ABCA4 (also known as ABCR or the rim protein) is a retinal-specific member of the ABCA subfamily predominantly expressed in the outer segment disk membranes of photoreceptor cells, and was the first ABCA transporter that has been linked to genetic disease. Available evidence suggested that ABCA4 may act as a flippase to translocate N-retinylidene-phosphatidylethanolamine (NRPE), a reversible covalent adduct of all-trans retinal (ATR) and phosphatidylethanolamine (PE), from the luminal leaflet to the cytoplasmic leaflet of the disk membrane. Here, we show the molecular structures of human ABCA4 determined in three distinct functional states by single-particle cryo-EM to 3.3–3.4 Å. These structures delineate the conformational transitions of ABCA4 to flip NRPE and suggest a “lateral access and extrusion” mechanism for ABCA4-mediated NRPE recognition and translocation, a mechanism that might also be adopted by other ABCA transporters.

To visualize ATP-driven conformational rearrangements of ABCA4, we characterized the structure of ABCA4QQ, a mutation that abolished ATP hydrolysis but maintained ATP binding, in the presence of 10 mM ATP/Mg2+. The structure was resolved at an overall resolution of 3.3 Å, showing excellent side-chain density for most of the protein except the lid and RD regions. Two strong and well-defined EM densities were observed for two bound ATP-Mg2+ molecules that were sandwiched between the two NBDs. The two NBDs exhibit a typical “head-to-tail” configuration predicted for all ABC transporters, forming two ATP binding-sites between the Walker A motif of one NBD and the ABC signature motif of the other NBD. The V-shaped lateral-opening conformation of the TMDs in the nucleotide-free ABCA4 structures is completely altered upon NBD dimerization induced by ATP binding. The two TMDs in the ATP-bound state form a closed conformation owing to the extensive interactions between TMs 1/2/5 and TMs 7/8/11, in contrast to a narrow interface in the cytoplasmic membrane leaflet between TM5 and TM11 in the nucleotide-free state. In the ATP-bound state, the NRPE and phospholipid-binding cavities in both membrane leaflets have been completely collapsed, with no space for bound molecules. The S-loop, which participates in NRPE substrate recognition in the nucleotide-free state, was not resolved in the ATP-bound state, suggesting the intrinsic flexibility of the S-loop during the transport cycle. After ATP binding, the ECD exhibits an obvious rotation toward the membrane, with a displacement for ~20 Å observed at the far end of the tunnel region. Our study also suggests that ATP binding might be sufficient for the NRPE-extrusion step and that ATP hydrolysis might be required to reset the transporter to the lateral-opening conformation ready for the next transport cycle.

> MADYKDDDDKSGPDEVDASGRMGFVRQIQLLLWKNWTLRKRQKIRFVVELVWPLSLFLVLIWLRNANPLYSHHECHFPNKAMPSAGMLPWLQGIFCNVNNPCFQSPTPGESPGIVSNYNNSILARVYRDFQELLMNAPESQHLGRIWTELHILSQFMDTLRTHPERIAGRGIRIRDILKDEETLTLFLIKNIGLSDSVVYLLINSQVRPEQFAHGVPDLALKDIACSEALLERFIIFSQRRGAKTVRYALCSLSQGTLQWIEDTLYANVDFFKLFRVLPTLLDSRSQGINLRSWGGILSDMSPRIQEFIHRPSMQDLLWVTRPLMQNGGPETFTKLMGILSDLLCGYPEGGGSRVLSFNWYEDNNYKAFLGIDSTRKDPIYSYDRRTTSFCNALIQSLESNPLTKIAWRAAKPLLMGKILYTPDSPAARRILKNANSTFEELEHVRKLVKAWEEVGPQIWYFFDNSTQMNMIRDTLGNPTVKDFLNRQLGEEGITAEAILNFLYKGPRESQADDMANFDWRDIFNITDRTLRLVNQYLECLVLDKFESYNDETQLTQRALSLLEENMFWAGVVFPDMYPWTSSLPPHVKYKIRMDIDVVEKTNKIKDRYWDSGPRADPVEDFRYIWGGFAYLQDMVEQGITRSQVQAEAPVGIYLQQMPYPCFVDDSFMIILNRCFPIFMVLAWIYSVSMTVKSIVLEKELRLKETLKNQGVSNAVIWCTWFLDSFSIMSMSIFLLTIFIMHGRILHYSDPFILFLFLLAFSTATIMLCFLLSTFFSKASLAAACSGVIYFTLYLPHILCFAWQDRMTAELKKAVSLLSPVAFGFGTEYLVRFEEQGLGLQWSNIGNSPTEGDEFSFLLSMQMMLLDAAVYGLLAWYLDQVFPGDYGTPLPWYFLLQESYWLGGEGCSTREERALEKTEPLTEETEDPEHPEGIHDSFFEREHPGWVPGVCVKNLVKIFEPCGRPAVDRLNITFYENQITAFLGHNGAGKTTTLSILTGLLPPTSGTVLVGGRDIETSLDAVRQSLGMCPQHNILFHHLTVAEHMLFYAQLKGKSQEEAQLEMEAMLEDTGLHHKRNEEAQDLSGGMQRKLSVAIAFVGDAKVVILDQPTSGVDPYSRRSIWDLLLKYRSGRTIIMSTHHMDEADLLGDRIAIIAQGRLYCSGTPLFLKNCFGTGLYLTLVRKMKNIQSQRKGSEGTCSCSSKGFSTTCPAHVDDLTPEQVLDGDVNELMDVVLHHVPEAKLVECIGQELIFLLPNKNFKHRAYASLFRELEETLADLGLSSFGISDTPLEEIFLKVTEDSDSGPLFAGGAQQKRENVNPRHPCLGPREKAGQTPQDSNVCSPGAPAAHPEGQPPPEPECPGPQLNTGTQLVLQHVQALLVKRFQHTIRSHKDFLAQIVLPATFVFLALMLSIVIPPFGEYPALTLHPWIYGQQYTFFSMDEPGSEQFTVLADVLLNKPGFGNRCLKEGWLPEYPCGNSTPWKTPSVSPNITQLFQKQKWTQVNPSPSCRCSTREKLTMLPECPEGAGGLPPPQRTQRSTEILQDLTDRNISDFLVKTYPALIRSSLKSKFWVNEQRYGGISIGGKLPVVPITGEALVGFLSDLGRIMNVSGGPITREASKEIPDFLKHLETEDNIKVWFNNKGWHALVSFLNVAHNAILRASLPKDRSPEEYGITVISQPLNLTKEQLSEITVLTTSVDAVVAICVIFSMSFVPASFVLYLIQERVNKSKHLQFISGVSPTTYWVTNFLWDIMNYSVSAGLVVGIFIGFQKKAYTSPENLPALVALLLLYGWAVIPMMYPASFLFDVPSTAYVALSCANLFIGINSSAITFILELFENNRTLLRFNAVLRKLLIVFPHFCLGRGLIDLALSQAVTDVYARFGEEHSANPFHWDLIGKNLFAMVVEGVVYFLLTLLVQRHFFLSQWIAEPTKEPIVDEDDDVAEERQRIITGGNKTDILRLHELTKIYPGTSSPAVDRLCVGVRPGECFGLLGVNGAGKTTTFKMLTGDTTVTSGDATVAGKSILTNISEVHQNMGYCPQFDAIDELLTGREHLYLYARLRGVPAEEIEKVANWSIKSLGLTVYADCLAGTYSGGNKRKLSTAIALIGCPPLVLLDQPTTGMDPQARRMLWNVIVSIIREGRAVVLTSHSMEECEALCTRLAIMVKGAFRCMGTIQHLKSKFGDGYIVTMKIKSPKDDLLPDLNPVEQFFQGNFPGSVQRERHYNMLQFQVSSSSLARIFQLLLSHKDSLLIEEYSVTQTTLDQVFVNFAKQQTESHDLPLHPRAAGASRQAQDLEGSDEVDAVEGSHHHHHHHHHH N-[3-(4-chlorophenyl)oxetan-3-yl]-4-[(3S)-3-hydroxypyrrolidin-1-yl]benzamide | C20 H21 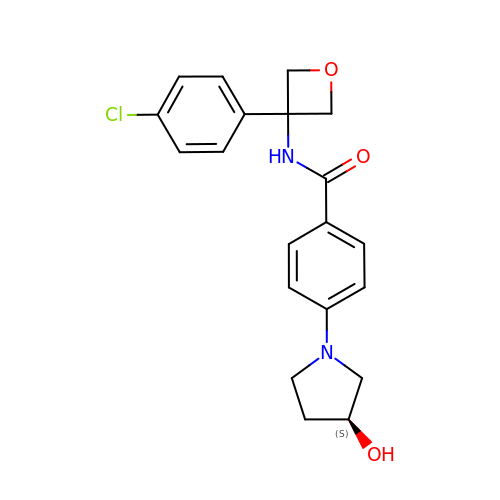Cl N2 O3 | XRPYHXDCSXOQDK-SFHVURJKSA-N> MGSHHHHHHHHHHSSGHLEVLFQGPSHMVDQATLDKLEAGFKKLQDATDCKSLLKKYLNREVFDQCKSLKTALGATLLDCIQSGVENLDSGVGIYAPDAEAYTLFAPIFNPIIEDYHEGFKPTDKHPPTDFGDINTIVNVDPSGKYVVSTHVRCGRSLKGYPFNPCLTEANYKEMEDKVSAIFGTFEGELKGKYYPLTGMDKATQQQLIDDHFLFKEGDRFLQAANACRYWPTGRGIYHNDAKTFLVWVNEEDHLRIISMQKGGDLKTIFQRLVNAV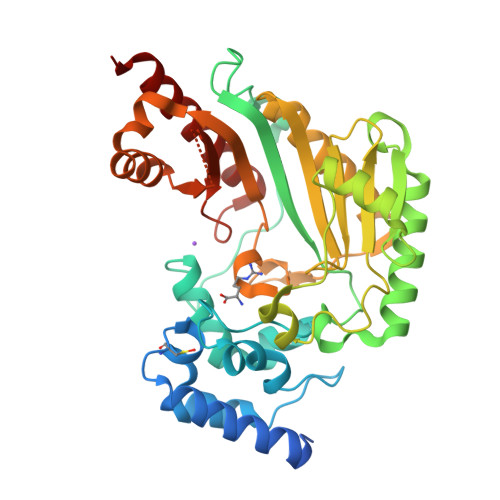NTIESKLPFSRDDRLGFLTFCPTNLGTTIRASVHIALPKLAKDKKQLEAIAAKFNLQVRGTRGEHTESEGGVYDISNKRRMGLTEYQAVKEMQDGILEMIKMEEAAP>[2x]MKNLRYKLLLFVFIGFWGLLALNLFILSVKNQEYYEKLAERNMTKKEFLVPTRGNITDRNDEFLATNELVFGVFLPSGLKQKDLLEKIEIIQKFFPNFSKETLLNNYQKENSLYNHNLIKVVGFIPYATMQPLYAKLIQTQGIFALPLDKRYYPNNALASHVLGYVGVASLQDLKDDEENQYSQIVGKTGIEKEYNKLLQGKVGYKIMRVNALNQELATLEVVLPSTNNHLQLSLDKRLQKEADKLFENKRGAILVMDAENGELLVAGSYPEYNLNDFVGGISQDKWQKLQDDIYNPLLNRFANALYPPGSVVKMGVGLSFLENLHITENTTIPTPPFIEVGKHKFRDWKKTGHGNSNLYKAIRESVDVYFYKFGLEISIEKLSKTLREVGFGEKTGVDLPNEFVGIVPDNLWKLKRFNQDWRVGDTLITAIGQGSFLATPLQVLAYTGLIATGKLATPHFAINNKQPLKDPLNSFQKKKLQALRVGMYEVCNHKDGTAYHSTRGSKITLACKTGTAQVVEIAQNIVNRMKEKDMEYFHRSHAWITAFLPYEKPKYAITILVEHGEGGSKLGGLLVKMSNKLYELGYLHHHHHH

Penicillin-binding proteins (PBPs) catalyze the two last reactions in PG biosynthesis (GlcNAc-MurNAc polymerization and stem peptide cross-linking, or transpeptidation). Class A enzymes can catalyze both reactions, while class B PBPs act uniquely as transpeptidases. Within the elongasome of a variety of bacteria including E. coli, Caulobacter crescentus, Bacillus subtilis, and Helicobacter pylori, PBPs have been shown to interact with, and be recruited by, the essential protein MreC, a bitopic membrane protein that is essential for cell shape. PBP2 (residues L38–L588, thus lacking the TM helix) is a 588-residue molecule that presents the characteristic fold of class B PBPs, with an elongated N-terminal region followed by a transpeptidase domain that carries the stem peptide cross-linking site.

The transpeptidase domain harbors the active site with the three conserved motifs: S–X–X–K (Ser311′–Val312′–Val313′–Lys314′), which includes the catalytic serine, located at the N-terminus of α2; S–X–N/D (Ser366′–Val367′–Asp368′), which lies between α4 and α5; and K–T/S–G (Lys513′–Thr514′–Gly515′), located at the C-terminus of β3 (PBP2 numbering indicated with a prime symbol). It is of note that a disulfide bond lies in the proximity of the active site, linking β3 to α9; a similar positioning for a disulfide bond in SpoVD (PBP2) from B. subtilis was recently linked to regulation of catalytic activity. Notably, in the crystal structure of unbound, closed PBP2, hydrophobic zipper residues Phe71′, Tyr127′, and Tyr134′ are covered by the anchor region, indicating that binding to MreC requires uncovering of this apolar patch through the swaying movement. A structure-based sequence comparison of class B PBPs from rod-like bacteria using the closed form of H. pylori PBP2 indicates that residues that line the head/anchor interface display clear similarities among class B enzymes. In addition, in structures of unbound class B PBPs from both Gram-positive and Gram-negative bacteria, analogous hydrophobic patches are covered by their respective anchor regions. In order to further characterize the “opening” mechanism of the N-terminal region of PBP2, we generated a “disulfide locked” form of PBP2 by engineering two cysteine residues at sites Tyr134′ and Ala218′, predicted to be well-positioned to form a disulfide bond. This mutant was unable to bind MreC in conditions where wild-type PBP2 could generate a stable complex in gel filtration.>FSPNNTNGSSTETVNSDIKTTTSSHPVSSLTMLNDTLHNIRTTNQALKKELSQKTLTKTSLEEIALHSSQISMDVNKSAQLLDILSRHEYPINKDARELLHSAPKEAELDGDQMISHRELWAK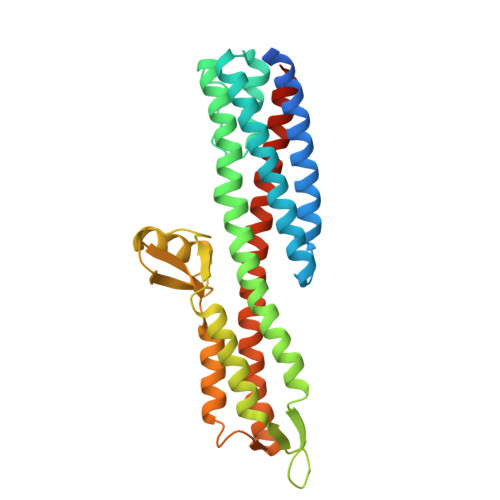IANSINDINEQYLKVYEHAVSSYTQMYQDFSAVLSSLAGWISPGGNDGNSVKLQVNSLKKALEELKEKYKDKPLYPANNTVSQEQANKWLTELGGTIGKVSQKNGGYVVSINMTPIDNMLKSLDNLGGNGEVVLDNAKYQAWNAGFSAEDETMKNNLQTLVQKYSNANSIFDNLVKVLSSTISSCTDTDKLFLHF[2x]> DQ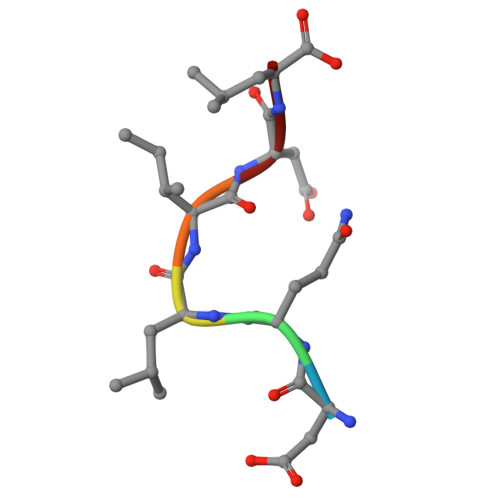LIDL>MDKYNNYSNVIKNKSSISPLLAAAAKIEPEITVLSSASKSNRSQYSQSLADTLLGLGYRSIFDIAKVSRQRFIKRHDESLLGNGAVIFDKAVSMANQVLQKYRKNRLEKSNSPLVPQTSSSTDASSESQTNKLPEYNQLFPEPWDNFCRPGAIEALDSPASYLLDLYKFIQSVELDGSNQARKLETRRADIPKLSLDNDALYKEVTALSIVNDVLSGSAREYIDQSGQADKAVNQILGDTHFPFTLPYSLPTQQINKGLGASNIELGTVIQRVDPQFSWNTTQEKYNQVLLAYTQLSSEQIALLSLPDVFTQNFLTQTELSAGYLSASTTEILAEKDLSRHGYIVKAADNIKGPTQLVEHSDASYDVIELTCTNQAKETITVKLRGENIITYQRTKARMVPFDNSSPFSRQLKLTFVAEDNPSLGNLDKGPYFANMDIYAAEWVRENVSSETMVSRPFLTMTYRIAIAKAGASLEELQPEADAFFINNFGLSAEDSSQLVKLVAFGDQTGSKAEEIESLLSCGENLPIVSPNVIFANPIFGSYFNDEPFPAPYHFGGVYINAHQRNAMTIIRAEGGREIQSLSNFRLERLNRFIRLQRWLDLPSHQLDLLLTSVMQADADNSQQEITEPVLKSLGLFRHLNLQYKITPEIFSSWLYQLTPFAVSGEIAFFDRIFNREQLFDQPFILDGGSFTYLDAKGSDAKSVKQLCAGLNISAVTFQFIAPLVQSALGLEAGTLVRSFEVVSSLYRLVSIPQTFGLSTEDGLILMNILTDEMGYLAKQPAFDDKQTQDKDFLSIILKMEALSAWLTKNNLTPASLALLLGVTRLAVVPTNNMVTFFKGIANGLSENVCLTTDDFQRQELEGADWWTLLSTNQVIDDMGLVLDIHPVWGKSDEEMLMEKIQSIGVSNDNNTLSIIVQILIQAKNAQENLLSQTISAEYGVERSVVPLQLRWLGSNVYSVLNQVLNNTPTDISSIVPKLSELTYSLLIYTQLINSLKLNKEFIFLRLTQPNWLGLTQPKLSTQLSLPEIYLITCYQDWVVNANKNEDSIHEYLEFANIKKTEAEKTLVDNSEKCAELLAEILAWDAGEILKAASLLGLNPPQATNVFEIDWIRRLQTLSEKTMISTEYLWQMGDLTENSEFSLKEGVGEAVMAALKAQGDSDNV[5x];>MSNSIEAKLQEDLRDALVDYYLGQIVPNSKDFTNLRSTIKNVDDLYDHLLLDTQVSAKVITSRLSLVTQSVQQYINRIALNLEPGLSINQQEATDWEEFANRYGYWAANQQLRMFPEIYVDPTLRLTKTEFFFQLESALNQGKLTDDVAQKAVLGYLNNFEEVSNLEIIAGYQDGIDIENDKTYFVARTRMQPYRYFWRSLDASQRNANSQELYPTAWSEWKAISVPLENVANGIVRPIMMDNRLYISWFEVAEEKETDSDGNIIVSGRYRTKIRLAHLGFDGVWSSGTTLREEVLADQMEEMIAVVDRMEDEPRLALVAFKEMSESWDVVFSYICDSMLIESSNLPTTTHPPKPGDGDKGLSDLDDYGANLVWFYLHETANGGKAEYKQLILYPVIINRDWPIELDKTHQGDFGTVDDFTLNSNYTGDELSLYLQSSSTYKYDFSKSKNIIYGIWKEDANNNRCWLNYKLLTPEDYEPQINATLVMCDKGDVNIITGFSLPNGGVDAGGKIKVTLRVGKKLRDKFQIKQFSQTQYLQFPEASSADVWYIGKQIRLNTLFAKELIGKASRSLDLVLSWETQNSRLEEAILGGAAELIDLDGANGIYFWELFFHMPFMVSWRFNVEQRYEDANRWVKYLFNPFECEDEPALLLGKPPYWNSRPLVDEPFKGYSLTQPSDPDAIAASDPIHYRKAVFNFLTKNIIDQGDMEYRKLQPSARTLARLSYSTASSLLGRRPDVQLTSFWQPLTLEDASYKTDSEIRAIEMQSQPLTFEPVVHDQTMSAVDNDIFMYPMNNELRGLWDRIENRIYNLRHNLTLDGKEINMDLYDSSISPRGLMKQRYQRVVTARNASKMNFKVPNYRFEPMLNRSKSGVETLIQFGSTLLSLLERKDSLSFDAYQMIQSGDLYRFSIDLQQQDIDINKASLEALQVSKQSAQDRYDHFKELYDENISSTEQKVIELQSQAANSLLMAQGMRTAAAALDVIPNIYGLAVGGSHWGAPLNAAAEIIMIKYQADSSKSESLSVSESYRRRRQEW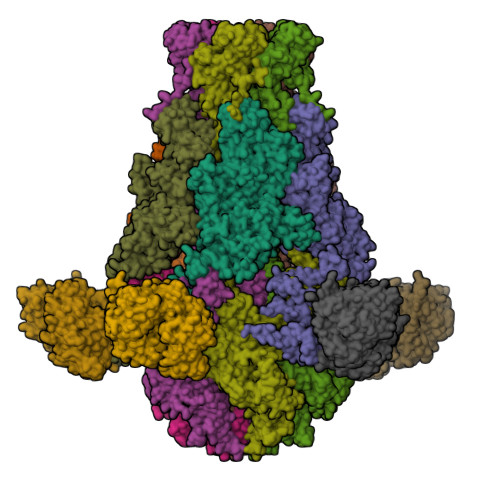ELQYKQAEWEVNSVEQQINLQNMQIKAANKRLEQVEAQQQQAMALLDYFSERFTNESLYTWLISQLSSLYLQAYDAVLSLCLSAEASLLYELNLGEQSFVGGGGWNDLYQGLMAGETLKLALMRMERVYVEQNSRRQEITKTISLKALLGESWPAELNKLKQKTPINFNLEEQIFVEDYQELYQRRIKSVSVSLPMLVGPYEDVCAQLTQTSSSYSTRADLKTVENMLTKRTFADTPHLVRSIQPNQQISLSTGVNDSGLFMLNFDDERFLPFEGSGVDSSWRLQFTNLKQNLDSLNDVILHVKYTAAIGSSTFSQGVRKILANINNDE[5x];>[5x]MVNKYTYTSSKAMSDISDVIGEPLAAWDSQVGGRVFNVIFDGKVYTNTYWVERWQVPGIGSSDGNPHNAWKFVRAATADEINKIGNPTTADVKPTENIPSPILVEDKYTEETYSRPDVNFKEDGSQGNLSYTATRVCAPMYNHYVGDKTKPKLSAYITDWCQYDARLDGGGSKEEERGRGFDLATLMQNPATYDRLIFSFLGICGDIGNKSKKVQEVWDGWNAQAPSLGLPQIGKGHIVPLDPYGDLGTARNVGLPPESADTSIESGTFLPYYQQNRAAGLLGGLRELQKKAHAMGHKLDLAFSIGGWSLSSYFSALAENPDERRVFVASVVDFFVRFPMFSCVDIDWEYPGGGGDEGNISSDKDGENYVLLIKELRSALDSRFGYSNRKEISIACSGVKAKLKKSNIDQLVANGLDNIYLMSYDFFGTIWADYIGHHTNLYSPKDPGEQELFDLSAEAAIDYLHNELGIPMEKIHLGYANYGRSAVGGDLTTRQYTKNGPALGTMENGAPEFFDIVKNYMDAEHSLSMGKNGFVLMTDTNADADFLFSEAKGHFISLDTPRTVKQKGEYAAKNKLGGVFSWSGDQDCGLLANAAREGLGYVADSNQETIDMGPLYNPGKEIYLKSISEIKSK>THPDISVDVLVIGAGPTGLGAAKRLNQIDGPSWMIVDSNETPGGLASTDVTPEGFLYDVGGHVIFSH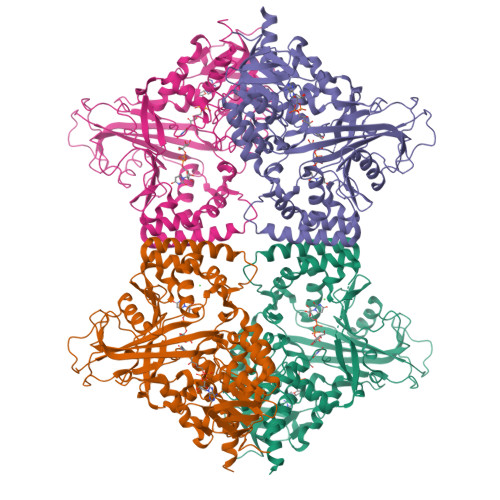YKYFDDCLDEALPKEDDWYTHQRISYVRCQGQWVPYPFQNNISMLPKEEQVKCIDGMIDAALEARVANTKPKTFDEWIVRMMGTGIADLFMRPYNFKVWAVPTTKMQCAWLGERVAAPNLKAVTTNVILGKTAGNWGPNATFRFPARGGTGGIWIAVANTLPKEKTRFGEKGKVTKVNANNKTVTLQDGTTIGYKKLVSTMAVDFLAEAMNDQELVGLTKQLFYSSTHVIGVGVRGSRPERIGDKCWLYFPEDNCPFYRATIFSNYSPYNQPEASKKLPTMQLADGSRPQSTEAKEGPYWSIMLEVSESSMKPVNQETILADCIQGLVNTEMLKPTDEIVSTYHRRFDHGYPTPTLEREGALTQILPKLQDKDIWSRGRFGSWRYEVGNQDHSFMLGVEAVDNIVNGAVELTLNYPDFVNGRQNTERRLVDGAQVFAKSKAQLELEHHHHHH[8x]>[2x]MTPMKTYDLIVIGTGPG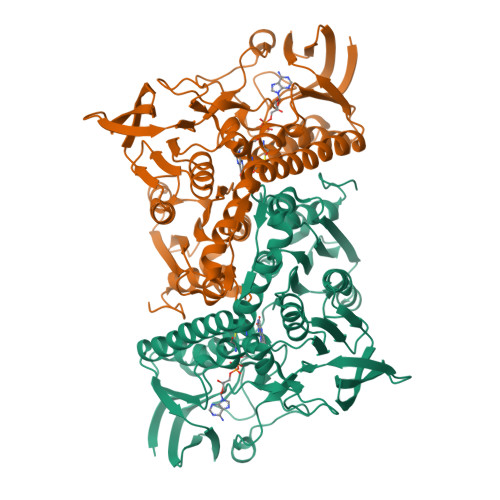GYHAAIRAAQLGLKVLAVEAGEVGGVCLNVGCIPTKALLHAAETLHHLKVAEGFGLKAKPELDLKKLGGWRDQVVKKLTGGVGTLLKGNGVELLRGFARLVGPKEVEVGGERYGAKSLILATGSEPLELKGFPFGEDVWDSTRALKVEEGLPKRLLVIGGGAVGLELGQVYRRLGAEVTLIEYMPEILPQGDPETAALLRRALEKEGIRVRTKTKAVGYEKKKDGLHVRLEPAEGGEGEEVVVDKVLVAVGRKPRTEGLGLEKAGVKVDERGFIRVNARMETSVPGVYAIGDAARPPLLAHKAMREGLIAAENAAGKDSAFDYQVPSVVYTSPEWAGVGLTEEEAKRAGYKVKVGKFPLAASGRALTLGGAEGMVKVVGDEETDLLLGVFIVGPQAGELIAEAALALEMGATLTDLALTVHPHPTLSESLMEAAEAFHKQAIHILNR> MDAYSTRPLTLSHGSLEHVLLVPTASFFIASQLQEQFNKILPEPTEGFAADDEPTTPAELVGKFLGYVSSLVEPSKVGQFDQVLNLCLTEFENCYLEGNDIHALAAKLLQENDTTLVKT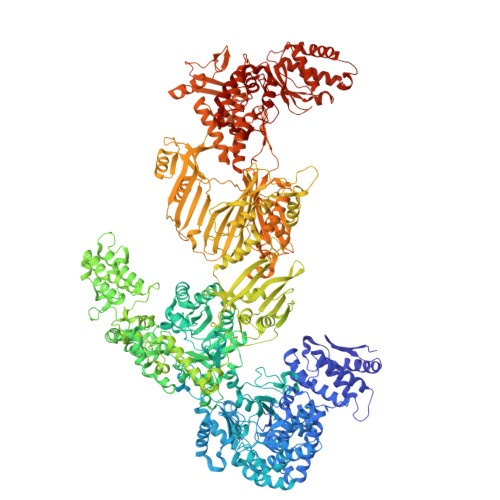KELIKNYITARIMAKRPFDKKSNSALFRAVGEGNAQLVAIFGGQGNTDDYFEELRDLYQTYHVLVGDLIKFSAETLSELIRTTLDAEKVFTQGLNILEWLENPSNTPDKDYLLSIPISCPLIGVIQLAHYVVTAKLLGFTPGELRSYLKGATGHSQGLVTAVAIAETDSWESFFVSVRKAITVLFFIGVRCYEAYPNTSLPPSILEDSLENNEGVPSPMLSISNLTQEQVQDYVNKTNSHLPAGKQVEISLVNGAKNLVVSGPPQSLYGLNLTLRKAKAPSGLDQSRIPFSERKLKFSNRFLPVASPFHSHLLVPASDLINKDLVKNNVSFNAKDIQIPVYDTFDGSDLRVLSGSISERIVDCIIRLPVKWETTTQFKATHILDFGPGGASGLGVLTHRNKDGTGVRVIVAGTLDINPDDDYGFKQEIFDVTSNGLKKNPNWLEEYHPKLIKNKSGKIFVETKFSKLIGRPPLLVPGMTPCTVSPDFVAATTNAGYTIELAGGGYFSAAGMTAAIDSVVSQIEKGSTFGINLIYVNPFMLQWGIPLIKELRSKGYPIQFLTIGAGVPSLEVASEYIETLGLKYLGLKPGSIDAISQVINIAKAHPNFPIALQWTGGRGGGHHSFEDAHTPMLQMYSKIRRHPNIMLIFGSGFGSADDTYPYLTGEWSTKFDYPPMPFDGFLFGSRVMIAKEVKTSPDAKKCIAACTGVPDDKWEQTYKKPTGGIVTVRSEMGEPIHKIATRGVMLWKEFDETIFNLPKNKLVPTLEAKRDYIISRLNADFQKPWFATVNGQARDLATMTYEEVAKRLVELMFIRSTNSWFDVTWRTFTGDFLRRVEERFTKSKTLSLIQSYSLLDKPDEAIEKVFNAYPAAREQFLNAQDIDHFLSMCQNPMQKPVPFVPVLDRRFEIFFKKDSLWQSEHLEAVVDQDVQRTCILHGPVAAQFTKVIDEPIKSIMDGIHDGHIKKLLHQYYGDDESKIPAVEYFGGESPVDVQSQVDSSSVSEDSAVFKATSSTDEESWFKALAGSEINWRHASFLCSFITQDKMFVSNPIRKVFKPSQGMVVEISNGNTSSKTVVTLSEPVQGELKPTVILKLLKENIIQMEMIENRTMDGKPVSLPLLYNFNPDNGFAPISEVMEDRNQRIKEMYWKLWIDEPFNLDFDPRDVIKGKDFEITAKEVYDFTHAVGNNCEDFVSRPDRTMLAPMDFAIVVGWRAIIKAIFPNTVDGDLLKLVHLSNGYKMIPGAKPLQVGDVVSTTAVIESVVNQPTGKIVDVVGTLSRNGKPVMEVTSSFFYRGNYTDFENTFQKTVEPVYQMHIKTSKDIAVLRSKEWFQLDDEDFDLLNKTLTFETETEVTFKNANIFSSVKCFGPIKVELPTKETVEIGIVDYEAGASHGNPVVDFLKRNGSTLEQKVNLENPIPIAVLDSYTPSTNEPYARVSGDLNPIHVSRHFASYANLPGTITHGMFSSASVRALIENWAADSVSSRVRGYTCQFVDMVLPNTALKTSIQHVGMINGRKLIKFETRNEDDVVVLTGEAEIEQPVTTFVFTGQGSQEQGMGMDLYKTSKAAQDVWNRADNHFKDTYGFSILDIVINNPVNLTIHFGGEKGKRIRENYSAMIFETIVDGKLKTEKIFKEINEHSTSYTFRSEKGLLSATQFTQPALTLMEKAAFEDLKSKGLIPADATFAGHSLGEYAALASLADVMSIESLVEVVFYRGMTMQVAVPRDELGRSNYGMIAINPGRVAASFSQEALQYVVERVGKRTGWLVEIVNYNVENQQYVAAGDLRALDTVTNVLNFIKLQKIDIIELQKSLSLEEVEGHLFEIIDEASKKSAVKPRPLKLERGFACIPLVGISVPFHSTYLMNGVKPFKSFLKKNIIKENVKVARLAGKYIPNLTAKPFQVTKEYFQDVYDLTGSEPIKEIIDNWEKYEQS>MEQEKVQELVSQMTLDEKIAQCLQLSPFLFKGTNKNAELTGPLLQEMKLTDAHTENAGSVLGSSSALDMIGIQEAYLKTNRLGIPLVFMADVIHGYKTVFPIPLALGCSFDRETVRVMAEVSALEATADGHHVTFSPMLDLVRDPRWGRVMESTGEDPFLNSELGKAMVDGYQGDASKLNENLEQMAACVKHFAAYGAAEAGLEYNTVNMSTRELYQNYLPAYNAAIQAGAKLVMTAFNVVDGIPATMNKWLNRDVLRGEMEFDGVLISAWGAVAEVINHGTARNPKEAAQFSMEAGVDLEMMTTCYIHELKGLIEEGKLSENLLDEAVLRMLNLKNDLGLFEDPYRGLKNNDRTKDILTDESRGKARAAGVESAVLLENKSRLLPLAKEAKIALVGPLATSPDILGGWNVYGEEKDGINVETGLREVFETVEVVSTEYTELSEEDKVAVKAAVQNMDVVVLALGEKNEWGGEAGSLATIRLPEAQYQLAKFVQTLGKPVVITLFNGRPLEVKELAESSDALLELWFPGTEAGRVTADLLSGASNPSGKLSMSFPQTTGQIPVYYNHLRTGRPQTPENKGERYVSHYLDIPNEPFYPFGYGKSYSEFELKTSSLPKELNLGESLHVEVTIKNISDIAGKEVIQVYLQDVTASISRPVKELKAFEKVALQAGEEKTVTFELTSEAFSFYNHQLEKVQEPGLHRVFVGTSSEDVDVFEVEVGGYVLEHHHHHH[2x]

In the gene cluster containing the lin1839 gene, the lin1840 gene encodes a putative glycoside hydrolase family (GH) 3 β-glucosidase (BGL) (GenBank accession number: CAC97071.1). The structure showed that Lin1840r forms a dimer of identical subunits each composed of three domains. The active center of Lin1840r is located at the interface of domains 1 and 2 as in the cases of known GH3 BGLs.

In the Cel2 and Gen2 complex structures, electron densities of Glc moieties were also both observed at subsite +1. These Glc moieties were thought to be the non-reducing ends of Cel2 and Gen2 due to the orientation of the hydroxy group participating in the glycosidic linkage, suggesting that Cel2 or Gen2 binds to the enzyme non-productively. In the both complexes, Glc molecules were observed only in molecule A. This might be due to impurity in quite high concentrations of soaked substrates. In the Cel2 complex, Trp409 stacks on another Glc moiety unlike in the cases of the Sop3 and Gen2 complexes. Unlike Lam2, Arg572 effectively excludes Cel2 as a substrate. However, the distance between Arg572 and the 6-OH of the glucoside in thioCel2 is so close as to cause steric hindrance. Actually, Cel2 binds to Lin1840r in the non-productive form. Moreover, the structure of the Lin1840r-Cel2 complex was compared with that of the JMB19063-Cel5 complex, which contains Glc in subsite −1 and Cel2 outside subsite −1. This complex is the same as the Cel2 complex of Lin1840r in that subsites +1 and −1 are filled with separate molecules.>[4x]GSPSRAEYRNWSKPQCDITGFAPFSKDNSIRLSAGGDI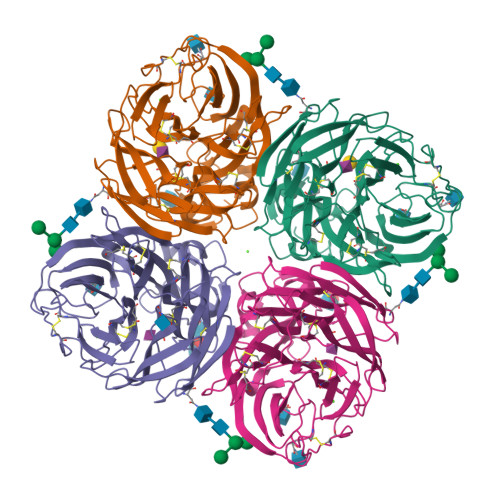WVTREPYVSCDPDKCYQFALGQGTTLNNVHSNNTVRGRTPYRTLLMNELGVPFHLGTKQVCIAWSSSSCHDGKAWLHVCITGDDKNATASFIYNGRLVDSVVSWSKEILRTQESECVCINGTCTVVMTDGSASGKADTKILFIEEGKIVHTSTLSGSAQHVEECSCYPRYPGVRCVCRDNWKGSNRPIVDINIKDHSIVSSYVCSGLVGDTPRKNDSSSSSHCLDPNNEEGGHGVKGWAFDDGNDVWMGRTINETSRLGYETFKVIEGWSNPKSKLQINRQVIVDRGNRSGYSGIFSVEGKSCINRCFYVELIRGRKEETEVLWTSNSIVVFCGTSGTYGTGSWPDGADLNLMPI>[18x]MS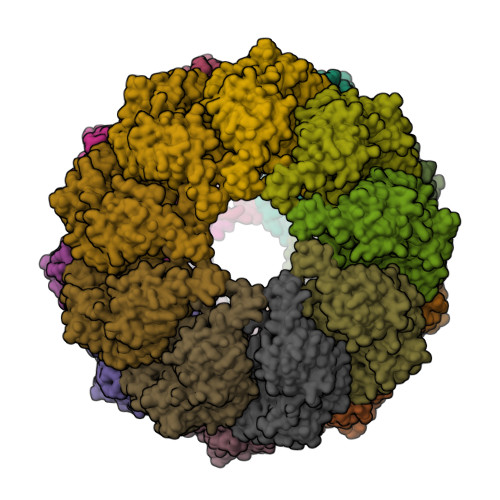SGVPVLLFKEGTSRNSGRDALKNNILAARTLAEMLRSSLGPKGLDKMLIDSFGDVTITNDGATIVKEMEIQHPAAKLLVEAAKAQDSEVGDGTTSAVVLAGLFLEKAESLVDQNIHPTIIIEGFKKAFNKSLELLPQLATKVDVSDLNSATARDALKKIVYTTMSSKFMAEGEELNKIMDIVIDAVTTVAEPLPDGGYNVSLDLIKIDKKKGGTIEDSQLIRGIVLDKEVVHAGMPRRVEKAKIAVLDASLEVEKPEISAKISITSPDQIKAFLDEEAKYLKDMVDKLASIGANVVICQKGIDDIAQHFLAKRGILAVRRVKRSDIEKLEKALGARIISSIKDATPEDLGYAELVEERKVGNDKMVFIEGAKNPKAVNILLRGSNDMALDEAERSINDALYSLRNILMEPYIVPGGGAIELELSARLREYARSVGGKEQLAIEAYADALEEIPMILAETAGLEPISALMDLRARHAKGLTNCGVDVINGKIIDDIYSINVVEPIRVTRQVLKSATEAATSIMKIDDLIAASQLKSSGKGAGAGAGGEGAEGGGAPSMEGLS>[6x]QGHMASMTGGQQMGRGSGPQKRCLFVCRHGERMDVVFGKYWLSQCFDAKGRYIRTNLNMPHSLPQRSGGFRDYEKDAPITVFGCMQARLVGEALLESNTIIDHVYCSPSLRCVQTAH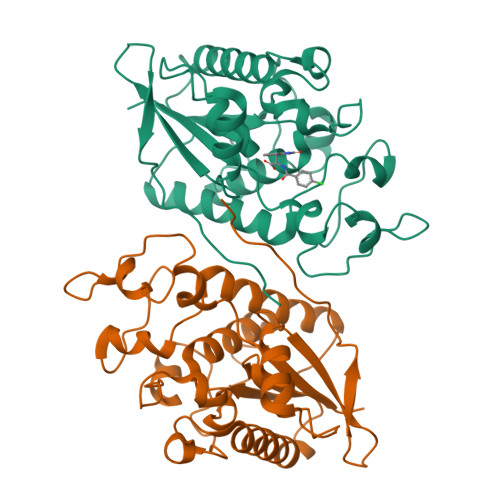NILKGLQQENHLKIRVEPGLFEWTKWVAGSTLPAWIPPSELAAANLSVDTTYRPHIPISKLVVSESYDTYISRSFQVTKEIISECKSKGNNILIVAHASSLEACTCQLQGLSPQNSKDFVQMVRKIPYLGFCSCEELGETGIWQLTDPPILPLTHGPTGGFNWRETLLQE>MSSTPSLSHSPAELYRAWQDLRAERPQLRARDAAALLQVSEGELVASRVGIDAVRLRPDWAALLPALGELGPIMALTRNEHCVHERKGPYREVTVSANGQMGLVVSPDIDLRLFLGGWNAVFAIAEETARGTQRSIQVFDQQGVAVHKVFLAEASDVRAWEPLVERLRAAEQDAVLALHEPRAPAAALVDAQIDAAALREGWAALKDTHHFHALLKKHGAQRTQALRLAGGEWAERLDNGDLAKLFEAAAESGLPIMVFVGNAHCIQIHTGPVCNLKWLDDWFNVLDPEFNLHLKTTGIAELWRVRKPSTDGIVTSWEAFDPDGELIVQLFGARKPGEPER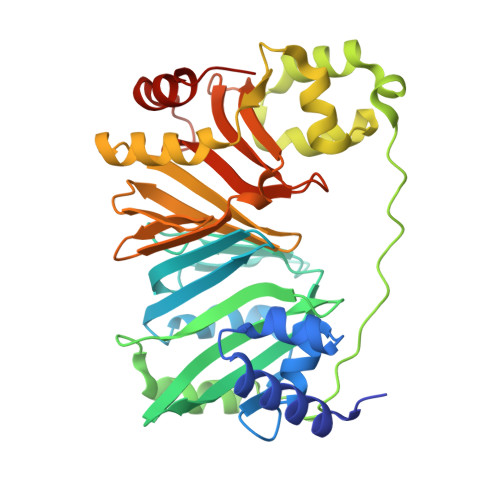DDWRELAESFKALHHHHHH[2x]Monoamine neurotransmitters such as serotonin and dopamine are loaded by vesicular monoamine transporter 2 (VMAT2) into synaptic vesicles for storage and subsequent release in neurons. VMAT2 inhibitors reserpine and tetrabenazine are used to treat hypertension, movement disorders associated with Huntington’s Disease and Tardive Dyskinesia. Here we present cryo-EM structures of human apo VMAT2 in addition to states bound to serotonin, tetrabenazine, and reserpine. These structures collectively capture three states, namely the lumen-facing, occluded, and cytosol-facing conformations.

We incubated VMAT2 with TBZ prior to vitrification, and obtained a 3.37 Å resolution VMAT2T map. A rod-like density in the central translocation funnel permits good fitting of a TBZ molecule, which was also supported by the overall stable molecular dynamics (MD) simulation trajectories. In our structure, VMAT2T adopts an occluded state, displaying concerted movements in the luminal halves of TM1, TM2, TM7, TM8 and TM10 compared with VMAT2A. Remarkably, beyond a rigid body rocking between the N- and C-domain, a unique transformation of helix-to-loop occurred at TM2 and TM7. Specifically, the last three helical turns (Residues 313–323) of TM7 unwound at Pro313 and stretched into an unstructured loop (LuL7–8), swinging towards TM1 and TM2 of the N-domain to block the luminal exit. Similarly, the luminal three helical turns of TM2 (Residues 124–132) unraveled from a hinge residue, Gly132, and ran along the newly exposed electronegative cleft after TM7’s relocation. This rearrangement latched the C-domain by buckling Leu124/Leu125 side-chains into a hydrophobic cavity occupied by TM7 apical residues Leu315 and Trp318. TBZ is situated just below the central plane of the translocation funnel. Its high binding affinity (60 nM) to VMAT2 corresponds to its occupation within an enlarged hydrophobic/electronegative pocket formed by TM1, TM2, TM4, TM5, TM7, TM8, TM10, and TM11. Mutational substitutions including Y341A, F429A, Y433A, I308A and I395A, had varying impacts on TBZ’s binding and inhibition activity against VMAT2. This robust non-polar network positions the sole tertiary amine of TBZ close to the negatively charged Glu312 on TM7. In the TBZ-bound VMAT2 structure, the carbonyl oxygen is oriented towards Asn34 on TM1.

> MALSELALVRWLQESRRSRKLILFIVFLALLLDNMLLTVVVPIIPSYLYSIKHEKNATEIQTARPVHTASISDSFQSIFSYYDNSTMVTGNATRDLTLHQTATQHMVTNASAVPSDCPSEDKDLLNENVQVGLLFASKATVQLITNPFIGLLTNRIGYPIPIFAGFCIMFVSTIMFAFSSSYAFLLIARSLQGIGSSCSSVAGMGMLASVYTDDEERGNVMGIALGGLAMGVLVGPPFGSVLYEFVGKTAPFLVLAALVLLDGAIQLFVLQPSRVQPESQKGTPLTTLLKDPYILIAAGSICFANMGIAMLEPALPIWMMETMCSRKWQLGVAFLPASISYLIGTNIFGILAHKMGRWLCALLGMIIVGVSILCIPFAKNIYGLIAPNFGVGFAIGMVDSSMMPIMGYLVDLRHVSVYGSVYAIADVAFCMGYAIGPSAGGAIAKAIGFPWLMTIIGIIDILFAPLCFFLRSPPSRLEEELRRRTEGGSSDLEVLFQ(2~{R})-2-(4-fluorophenyl)-~{N}-[4-[2-[(2-methoxy-4-methylsulfonyl-phenyl)amino]-[1,2,4]triazolo[1,5-a]pyridin-6-yl]phenyl]propanamide 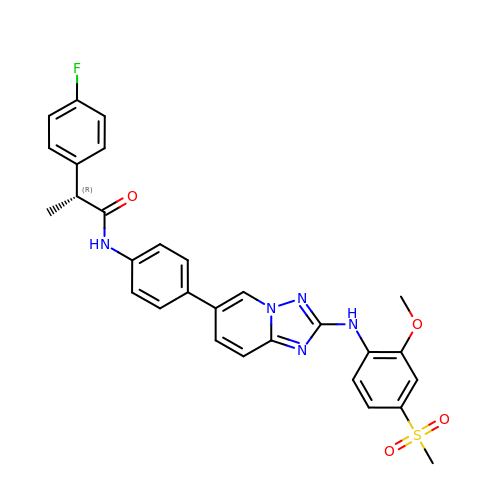| C29 H26 F N5 O4 S | NRJKIOCCERLIDG-GOSISDBHSA-N>MDLGLKDKVALITGSSAGIGFTIAEKLAEEGCHLIICGRNSQRLEQAYQSLAQAYPAQQILRLVADVHQAQDSEQLIQDSLNQYGKIDILVNNSEGANFAENLIENLSDEDWLNVFQGKLIGYIRLTNLVLPIMKKQHWGRIVNIIGTSGKEPSPRLVKSGVVNAALMNFTKSVARQTAPYNVLINSVNPGVIDTPRHREYLEIYAKKEGTTPDLIRERILKTIPMNRIGTTEEFANLVVFLASECASYITGITIPLDG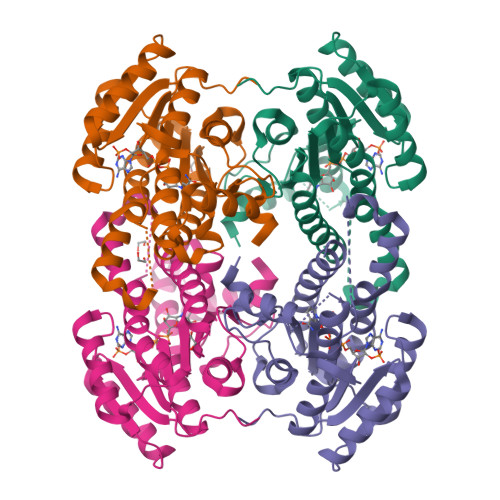GLSSSAFLEHHHHHH[2x]>[2x]GSMAPRAGFDAEQVRDKARKDLLHLLEGVRGKKNLVIEKDLAGPLGVIVKASTLRDYGVDNFFFLENKNTGTSQRNIVFIARGESVRNAHAIAAQIKRIQRESQTSHDFHIFWVPRRTLFSDKVLEEAGVLGDANISELPLYFFPLERDVLSLELNDSFRDLYLAKDPTPVFLLSRALMGIQKKHGLFPRIIGKGENAKRVADLLSRMRQELLAGEEAGESDRAGLSPSTTIESVIIIDREVDFVTPLLTQLTYEGLIDEYFGIQNNQTDVDAVIVGAPAQSAASTSTAVPTNSSQSRKRKIQLDGSDSLYSQLRDANFAIVGSLLNTVARRLKSDYESRHNTKTTAELKEFVKKLPGYQAEQQSLKIHSNIAEEIINYTRTEIFNKLLEVQQNLAAGADPSSQFDSIEELVARDTPLPQVLRLLCLYSCISGGIKTKELDHFRRLVLQGYGHQHLLTLHNLERLQMFLSKSSPLASMITMSGSSGGPDQKTNYTYLRKQLRLIVDEVNEQDPNDIAYVYSGYAPLSIRLVQCVLQKQYLLSITKGSGTVIAAGPVAGGGAQGWKGFEEIVKHARGPTFDEIQKGEDKAVKARALLSGSSGDKKTVFVVFVGGITFTEIAALRFIAKQEEARRNIVICTTSIINGNRMMNAAIETATFEKTTVTTAAAQ

Vps33 regulates fusion in the endo-lysosomal membrane system as a stable subunit within two large multisubunit tethering complexes, HOPS (homotypic fusion and vacuolar protein sorting) and CORVET (class C core vacuole/endosome tethering). Vps33 shares the overall shape and topology observed for previously reported SM protein structures. Following the nomenclature introduced by Misura et al., Vps33 contains three domains: domain 1 (residues 1–138; red), domain 2 (residues 139–248 and 502–667; green), and domain 3 (residues 249–501; blue), with domain 3 further subdivided into 3a (residues 249–380) and 3b (residues 381–501). The C. thermophilum Vps33 and Vps16CTD–Vps33 structures provide a first detailed view of an SM protein from the Vps33 family and of its recruitment into a multisubunit tethering complex.

The structure of C. thermophilum Vps33 was determined using MAD phasing and refined to 2.6 Å resolution. The two copies of Vps33 present within each asymmetric unit of the crystal are highly similar to one another and can be superimposed with a root-mean-squared deviation of only 0.56 Å (over 580 Cα atoms). Despite this very high degree of overall similarity, a functionally important region of domain 3a adopts somewhat different conformations in the two Vps33 monomers. Within our Vps33-only crystals, the tip of domain 3a adopts two different open conformations dictated by direct, intermolecular tip-tip interactions within each asymmetric unit. The positioning of domain 1 in Vps33 is substantially different from that observed in all previously determined SM protein structures. For example, after domains 2 and 3 of the two independent copies of monomeric Vps33 are superimposed, the two copies of domain 1 differ by only a 2.2° rotation and a 0.6 Å translation. Our Vps33 structure, the first of a class II SM protein, makes it clear why Vps33 is unable to bind N-peptides. The structural basis for this key distinction among SM protein families can be understood by superimposing domain 1 of Vps33 upon that of other, N-peptide-binding SM proteins. This analysis reveals that the binding site normally occupied by the N-peptide’s conserved Arg side chain is, uniquely in the case of Vps33, filled by Arg-115 of the SM protein itself. In this case a displacement of the Vps33 backbone, relative to other SM proteins, causes the side chain of Leu-129 to occupy the binding pocket. Thus, both of the pockets that in other SM proteins accommodate conserved Qa-SNARE N-peptide residues are missing in Vps33.>[2x]MKIGIIGAGQLARMLSLAGTPLGLEFHCLGKNGDCAEEVVKTVTDIELTKVNDVVAWAKQFDVITFENENISHELIKAINHEVSVYPSAKAIAISQDRLLEKSFMQDHGIATAKFVNIDSLAKLQSAVDDHGLPAILKTRRFGYDGKGQFVIRSQEDITKAWDVLKDAPDGLIYEAFVDFDYEVSQICTADLKGNIAFYPLARNTHKQGIIVESEAPFENVV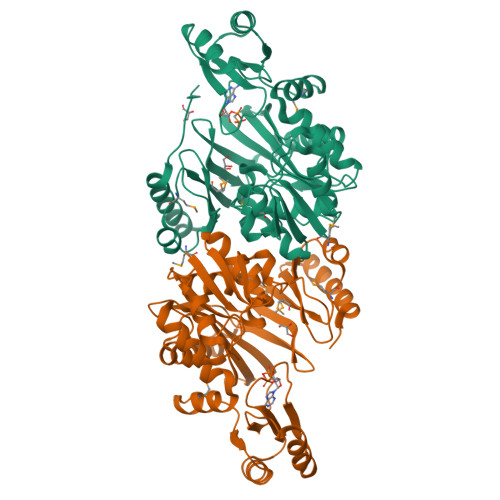LAEKAQQIAKILVKEFAYVGTLAIEFFVKGDELIVNEIAPRVHNSGHWSIDGAVTSQFENHVRAIAGLILGDTTSRKTVMLNCIGGMPATKDLAALDRVKIHSYNKEPRKGRKVGHLNLNLNDETDEYQLLQVKKLIALSEEIAGENLYFQ>MSSNDSAQTRNLQEERFNERTSTPTVVTAVLPDTNGPTTNSTSGSVGPPHPTPNVPVPTQSSSDPPSASGIFAKEIDLPRNVIQHSGNKFILDVVPDSRFPTFAITEFVQRSFSNFTFEQYSYVSPASLVGYLVYMIHAFVFLVDAFERSPMSAYASEIDASHAYLRIIDAFSDAYIPDFLFEILDTYLSHRLDIRSKLEMNVSYGSVLYKYDAPRIVAPSIFLLAHNQLISQSRESTAYEKWLDSIVIHYSRAVIRVGNLVGGLYQSSHGSTTTHFTYRNWFARSLSRLADSATHRTHLRRPMISEFDYNIPSVNNNTYNPYVHLLMLEPNNRNITLDFIRSLSSFCSTELKATRTLRDHISRRSAAISRCVIKGPEAPTWHSSPLDDLKEKSKQGNFSQFCEVAKFGLPRKENSESYTFKFPKDASTIDTAFYLIQENGRSSVLDPTTADEELHTEGMNLLFDPYDDESSAHYATVLSGKLIQNSNIDGETLLLPDPTTGLARTNSRYLQGSVLIRNVLPEFDQHEIRLFPRYPQISRLSASLTLLFNMRQVWIPRFKQKVDEQPKLSNFSWNEGCDGTVPSLNVVTAESSTNGPAAEQQVILWSSYRHVSNSDRPTVDTVYYYSTLELLFGTRSSMMQ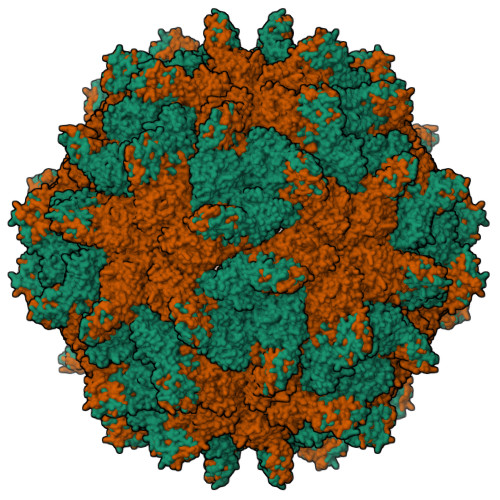TYNLHQLLSLH[2x]(2S)-N,2-dicyclohexyl-2-{2-[4-(hydroxymethyl)phenyl]-1H-benzimidazol-1-yl}acetamide | C28 H35 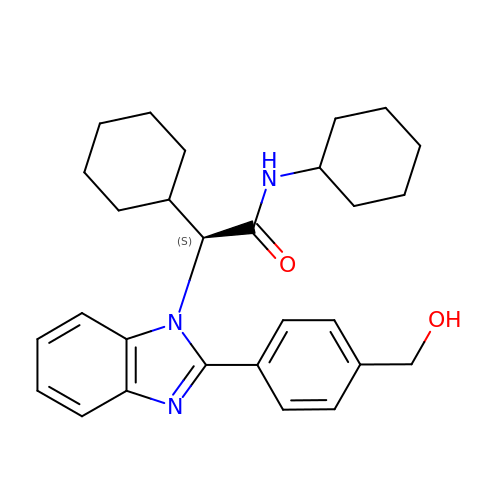N3 O2 | VNQAIQZVCULCDE-SANMLTNESA-N>ALETLAFDGRTYIEYLNAVIESELTNEIPAEKAL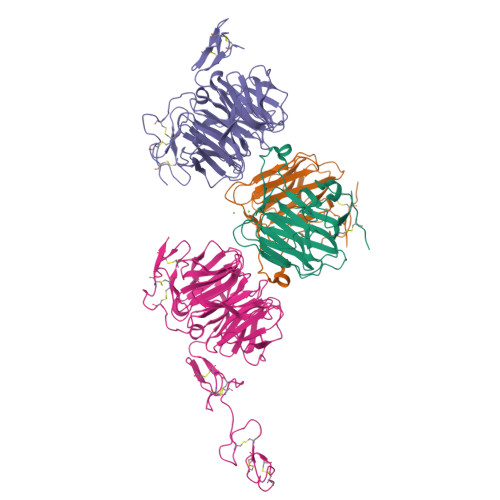QSNHFELSLRTEATQGLVLWIGKAAERADYMALAIVDGHLQLSYDLGSQPVVLRSTVKVNTNRWLRIRAHREHREGSLQVGNEAPVTGSSPLGATQLDTDGALWLGGLQKLPVGQALPKAYGTGFVGCLRDVVVGHRQLHLLEDAVTKPELRPCPTP[2x];>TGEENCNVNNGGCAQKCQMIRGAVQCTCHTGYRLTEDGRTCQDVNECAEEGYCSQGCTNSEGAFQCWCEAGYELRPDRRSCKALGPEPVLLFANRIDIRQVLPHRSEYTLLLNNLENAIALDFHHRRELVFWSDVTLDRILRANLNGSNVEEVVSTGLESPGGLAVDWVHDKLYWTDSGTSRIEVANLDGAHRKVLLWQSLEKPRAIALHPMEGTIYWTDWGNTPRIEASSMDGSGRRIIADTHLFWPNGLTIDYAGRRMYWVDAKHHVIERANLDGSHRKAVISQGLPHPFAITVFEDSLYWTDWHTKSINSANKFTGKNQEIIRNKLHFPMDIHTLHPQRQPAGKNRCGDNNGGCTHLCLPSGQNYTCACPTGFRKINSHACAQ[2x]> GSHHHHHHSS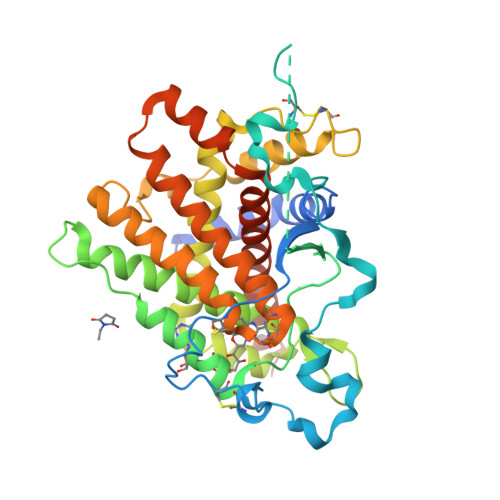GLVPRGSFNELNAINENIRDDLSALLKSDFFKYFRLDLYKQCSFWDANDGLCLNRACSVDVVEDWDTLPEYWQPEILGSFNNDTMKEADDSDDEAKFLDQLCQTSKKPVDIEDTINYADVNDFNGKNAVLIDLTANPERFTGYGGKQAGQIWSTIYQDNCFTIGETGESLAKDAFYRLVSGFHASIGTHLSKEYLNTKTGKWEPNLDLFMARIGNFPDRVTNMYFNYAVVAKALWKIQPYLPEFSFCDLVNKEIKNKMDNVISQLDTKIFNEDLVFANDLSLTLKDEFRSRFKNVTKIMDCVQCDRCRLWGKIQTTGYATALKILFEINDADEFTKQHIVGKLTKYELIALLQTFGRLSESIESVNMFEKMYGKRLLERPHRD Recently, we have successfully expanded the scope of available synthetic metal complexes for heme substitution in the heme acquisition system protein A (HasAp)16–21 which is a hemophore secreted by Pseudomonas aeruginosa under iron-deficient conditions. Herein, we report a heme-substituted protein dimer composed of the native hemoprotein HasA, which accommodates a tetraphenylporphyrin bearing an additional metal coordination site. Herein we report the dimerization of HasApf5 derived from Pseudomonas protegens PF-5,34 by incorporating Fe-TPP with a phenanthroline (phen) ligand as an additional metal coordination site. By the addition of Ni2+ ions, HasApf5 binds Fe-TPP-phen to form a stable dimer structure with a bent configuration.

To explore the types of metal complexes that could be incorporated into HasA originated from bacteria having the heme acquisition system, we found that HasApf5, derived from Pseudomonas protegens PF-5, can form a more stable complex with Fe-TPP than HasAp. Size-exclusion chromatography (SEC) analysis of HasApf5 bound to Fe-TPP showed a single sharp peak under both alkaline and neutral conditions (pH 7.0–9.5), whereas Fe-TPP bound to HasAp gave a single sharp peak only under alkaline conditions. The UV-vis spectra of HasApf5 bound to Fe-TPP recorded after several days were almost identical to the initial spectra even under neutral conditions (Fig. S2†), suggesting that the Fe-TPP binding is highly stable. Furthermore, HasApf5 capture of Fe-TPP was stable even at high temperatures. The Tm value of HasApf5 capture of Fe-TPP was estimated to be 60.5 °C, which is relatively high and comparable to that of HasAp-bound Fe-TPP under alkaline conditions (62.4 °C) (Table S1†). The crystal structure of HasApf5 with Fe-TPP was determined at 1.45 Å resolution. Its overall structure is similar to that of HasAp with Fe-TPP (root-mean-square deviation [RMSD] over amino acid residues 2–180 for Cα atoms: 0.397), and Fe-TPP is positioned in the heme-binding site with coordination by His32 and Tyr75. Upon closer examination and comparison, additional hydrogen bonds mediated by water molecules were observed at the Fe-TPP binding site: namely, Glu36-water-Arg33, Lys124-water-Ser79 and -Asn80. These additional hydrogen-bonding interactions appear to contribute to the stabilization of the Fe-TPP binding. The result of docking simulations of Fe- TPP-phen into HasApf5 using the crystal structure of the Fe-TPP-binding form indicated that the phen ligand is anchored away from the HasApf5 surface, suggesting that the formation of HasApf5 assemblies would be possible through the addition of metal ions.

>[2x]GSMSISISYSATYGGNTVAQYLTDWSAYFGDVNHRPGEVVDGTNTGGFNPGPFDGTQYAIKSTASDAAFVADGNLHYTLFSNPSHTLWGSVDTISLGDTLAGGSGSNYNLVSQEVSFTNLGLNSLKEEGRAGEVHKVVYGLMSGDSSALAGEIDALLKAIDPSLSVNSTFDDLAAAGVAHVNPAA>[2x]RE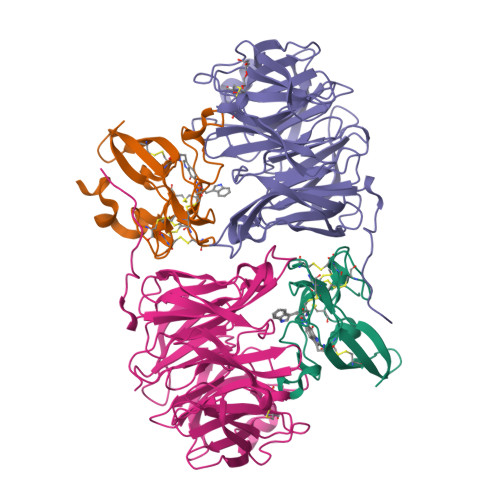VLTGGHSVSAPQENRIYVMDSVFMHLTESRVHVYDYTNGKFLGMVPTAFNGHVQVSNDGKKIYTMTTYHERITRGKRSDVVEVWDADKLTFEKEISLPPKRVQGLNYDGLFRQTTDGKFIVLQNASPATSIGIVDVAKGDYVEDVTAAAGCWSVIPQPNRPRSFMTICGDGGLLTINLGEDGKVASQSRSKQMFSVKDDPIFIAPALDKDKAHFVSYYGNVYSADFSGDEVKVDGPWSLLNDEDKAKNWVPGGYNLVGLHRASGRMYVFMHPDGKEGTHKFPAAEIWVMDTKTKQRVARIPGRDALSMTIDQQRNLMLTLDGGNVNVYDISQPEPKLLRTIEGAAEASLQVQFHPVGGT;>[2x]AGGGGSSSGADHISLNPDLANEDEVNSCDYWRHCAVDGFLCSCCGGTTTTCPPGSTPSPISWIGTCHNPHDGKDYLISYHDCCGKTACGRCQCNTQTRERPGYEFFLHNDVNWCMANENSTFHCTTSVLVGLAKN THIOBUTYRIC ACID S-{2-[3-(2-HYDROXY-3,3-DIMETHYL-4-PHOSPHONOOXY-BUTYRYLAMINO)-PROPIONYLAMINO]-ETHYL} ESTER | C15 H29 N2 O8 P 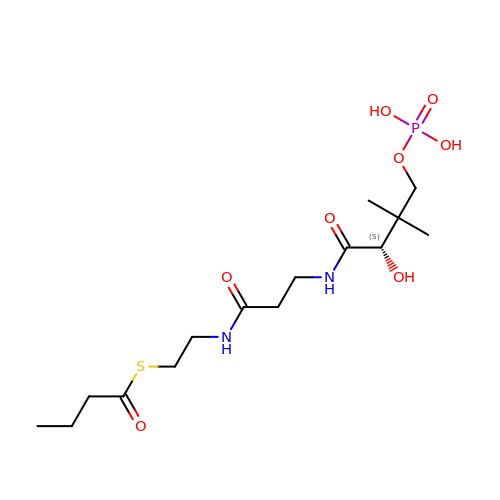S | PZIQDUSGQUZEBS-CYBMUJFWSA-N> MGRLLALVVGAALVSSACGGCVEVDSETEAVYGMTFKILCISCKRRSETNAETFTEWTFRQKGTEEFVKILRYENEVLQLEEDERFEGRVVWNGSRGTKDLQDLSIFITNVTYNHSGDYECHVYRLLFFENYEHNTSVVKKIHIEVVDKANRDMASIVSEIMMYVLIVV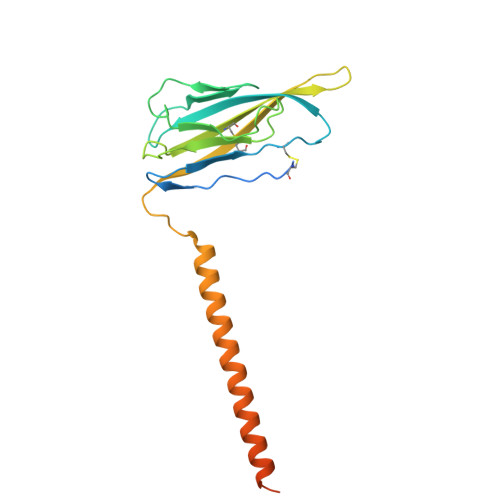LTIWLVAEMIYCYKKIAAATETAAQENASEYLAITSESKENCTGVQVAE> MGAGEKGIVEKEGYQLDTRRQAQAAYPRIKVLVIHYTADDFDSSLATLTDKQVSSHYLVPAVPPRYNGKPRIWQLVPEQELAWHAGISAWRGATRLNDTSIGIELENRGWQKSAGVKYFAPFEPAQIQALIPLAKDIIARYHIKPENVVAHADIAPQRKDDPGPLFPWQQLAQQGIGAWP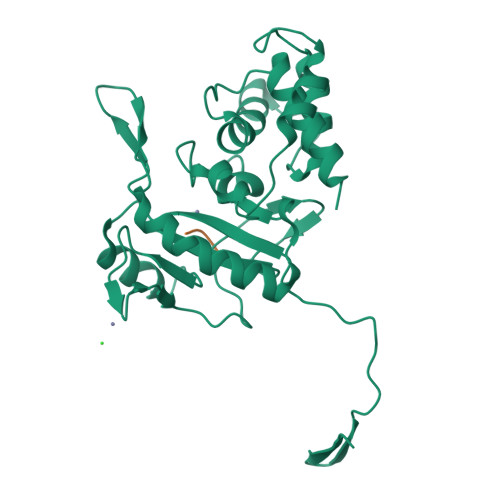DAQRVNFYLAGRAPHTPVDTASLLELLARYGYDVKPDMTPREQRRVIMAFQMHFRPTLYNGEADAETQAIAEALLEKYGQD;> AEK>MGSDKIHHHHHHMPKIWTERIFDDPEIYVLRIDDDRIRYFEAVWEIPEGISYNAYLVKLNGANVLIDGWKGNYAKEFIDALSKIVDPKEITHIIVNHTEPDHSGSLPATLKTIGHDVEIIASNFGKRLLEGFYGIKDVTVVKDGEEREIGGKKFKFVMTPWLHWPDTMVTYLDGILFSCDVGGGYLLPEILDDSNESVVERYLPHVTKYIVTVIGHYKNYILEGAEKLSSLKIKALLPGHGLIWKKDPQRLLNHYVSVAKGDPKKGKVTVIYDSMYGFVENVMKKAIDSLKEKGFTPVVYKFSDEERPAISEILKDIPDSEALIFGVSTYEAEIHPLMRFTLLEIIDKANYEKPVLVF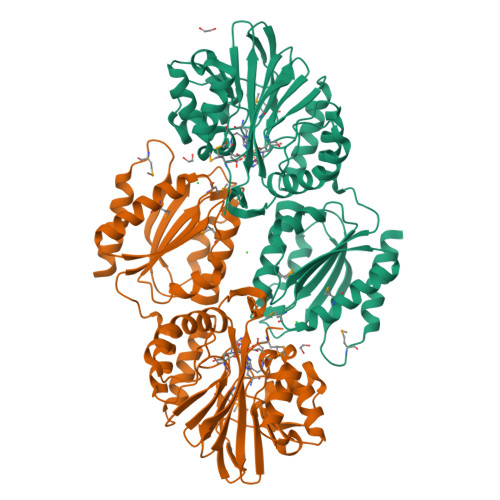GVHGWAPSAERTAGELLKETKFRILSFTEIKGSNMDERKIEEAISLLKKELE[2x]> ADGLYLQVGAFANPDAAELLKAKLSGVTAAPVFISSVVRNQQILHRVRLGPIGSAD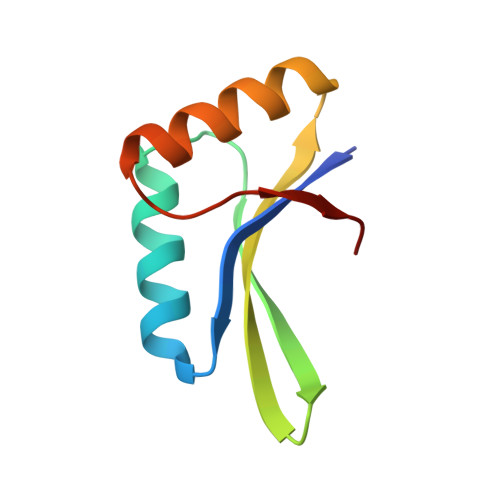EVSRTQDSIRVANLGQPTLVRPD> MESTANALVVKVSYGGVLRRFRVPVKANGQLDLEMAGLKEKIAALFNLSADAE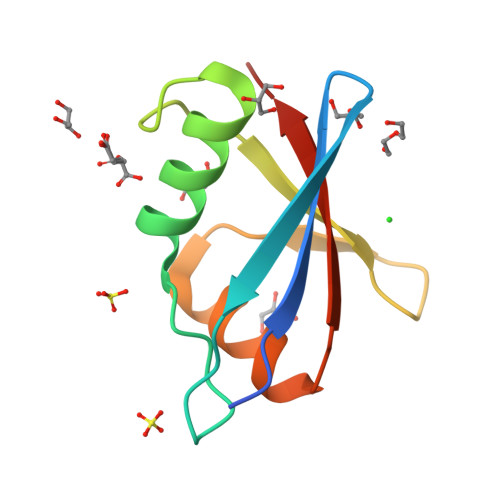LSLTYSAADGAVVALVDDNDLFDVTNQRLKFLKINVNAGVS>MGNRGMEDLIPLVNRLQDAFSAIGQNADLDLPQIAVVGGQSAGKSSVLENFVGRDFLPRGSGIVTRRPLVLQLVNATTEYAEFLHCKGKKFTDFEEVRLEIEAETDRVTGTNKGISPVPINLRVYSPHVLNLTLVDLPGMTKVPVGDQPPDIEFQIRDMLMQFVTKENCLILAVSPANSDLANSDALKVAKEVDPQGQRTIGVITKLDLMDEGTDARDVLENKLLPLRRGYIGVVNRSQKDIDGKKDITAALAAERKFFLSHPSYRHLADRMGTPYLQKVLNQQLTNHIRDTLPGLRNKLQSQLLSIEKEVEEYKNFRPDDPARKTKALLQMVQQFAVDFEKRIEGSGDQIDTYELSGGARINRIFHERFPFELVKMEFDEKELRREISYAIKNIHGIRTGLFTPDMAFETIVKKQVKKIREPCLKCVDMVISELISTVRQCTKKLQQYPRLREEMERIVTTHIREREGRTKEQVMLLIDIELAYMNTNHEDFIGFANAQQRSNQMNKKKTSGNQDEILVIRKGWLTINNIGIMKGGSKEYWFVLTAENLSWYKDDEEKEKKYMLSVDNLKLRDVEKGFMSSKHIFALFNTEQRNVYKDYRQLELACETQEEVDSWKASFLRAGVYPERVGDKEKASETEENGSDSFMHSMDPQLERQVETIRNLVDSYMAIVNKTVRDLMPKTIMHLMINNTKEFIFSELLANLYSCGDQNTLMEESAEQAQRRDEMLRMYHALKEALSIIGDINT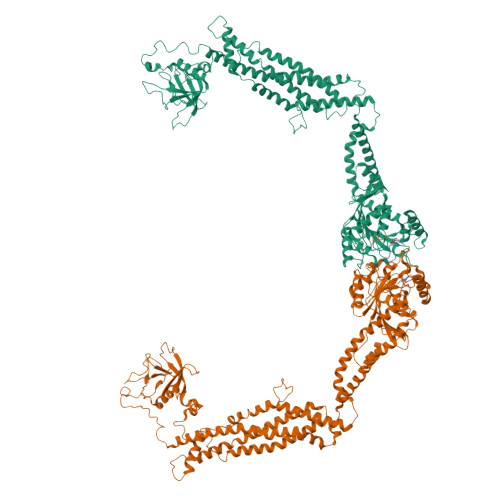T[2x]Here we focus on the prokaryotic Argonaute AfAgo from Archaeoglobus fulgidus DSM4304. Although phylogenetically classified as a long-B pAgo, AfAgo contains only MID and catalytically inactive PIWI domains, akin to short pAgos. We show that AfAgo forms a heterodimeric complex with a protein encoded upstream in the same operon, which is a structural equivalent of the N-L1-L2 domains of long pAgos. This complex, structurally equivalent to a long PAZ-less pAgo, outperforms standalone AfAgo in guide RNA-mediated target DNA binding.

Comparison of this 172 aa ORF to a homologous sequence found in a nearly identical AfAgo-encoding genetic island present in the genome of a related strain A. fulgidus DSM88774 revealed that it contains a premature STOP codon due to a 2 bp deletion. To study the structure and function of the full-length upstream protein, the restored full-length open reading frame, with the missing TA nucleotides inserted, was cloned into an E. coli expression vector and the corrected protein was subsequently purified by liquid chromatography. We were able to solve its structure by X-ray crystallography in two symmetry groups: P1 (resolution 1.85 Å) and P3221 (resolution 1.4 Å). Two full-length upstream protein chains found in the asymmetric unit of the P1 structure, and a single chain found in the asymmetric unit of the P3221 structure overlap with an RMSD of 0.85 Å (determined using PDBe Fold). We henceforth refer to the full-length upstream protein as AfAgo-N. The upstream protein (AfAgo-N) is the structural equivalent of the N-L1-L2 domains of long pAgo proteins.

>[2x]MGSSHHHHHHSQDPMEIPLSSGNVNTPDVRSSGILYINIYPIVNYPETIKVSAIPYYEEFLPGKWKKRIGDLIYLYGYGIENEFDEIDNSNALFGKIFRKYLLDILSENIATPWQLKELGSTLRLVKEITENYEFSNIIKLQYELIINVHHWQNTNFGIIVDLKINILDRENNQRISYTKIKDKYGESVKKKIWVSVQAFHRHLTPEGKKYATAMRDKFNLLTGLLKEAFGSSEDEKTFSTPDGEIKIVFKPLEIVEVSNNDGI> AKTEPSEKSVEIMRKFSEQYARRSGTYFCVDKGVTSVVIKGLAEHKDSYGAPLCPCRHYDDKAAEVGQGFWNCPCVPMRERKECHCMLFLTPDNDFAGKDQTITSDEIKETTANM;> IE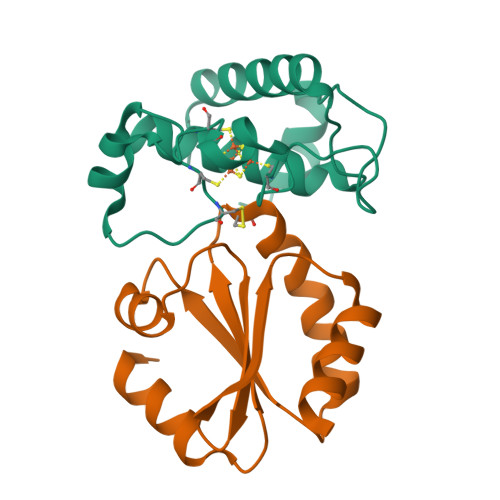AKKQTFDSFEDLLVNSDKPVLVDYYATWCGPSQFMVPILNEVSETLKDKIQVVKIDTEKYPSIANKYKIEALPTFILFKDGEPCDRFEGALTAKQLIQRIEDSLKVKP>[2x]MEEPEEPADSGQSLVPVYIYSPEYVSMCDSLAKIPKRASMVHSLIEAYALHKQMRIVKPKVASMEEMATFHTDAYLQHLQKVSQEGDDDHPDSIEYGLGYDCPATEGIFDYAAAIGGATITAAQCLIDGMCKVAINWSGGWHHAKKDEA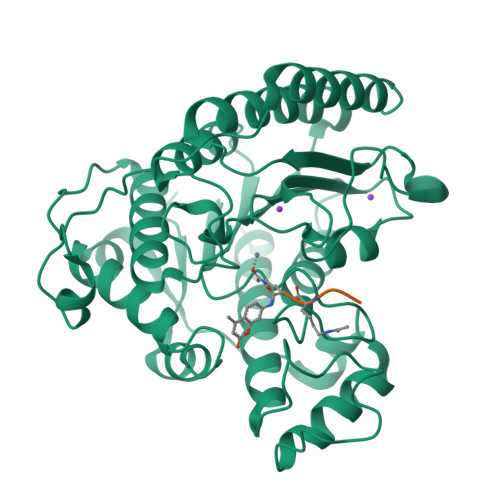SGFCYLNDAVLGILRLRRKFERILYVDLDLHHGDGVEDAFSFTSKVMTVSLHKFSPGFFPGTGDVSDVGLGKGRYYSVNVPIQGGIQDEKYYQICESVLKEVYQAFNPKAVVLQLGADTIAGDPMCSFNMTPVGIGKCLKYILQWQLATLILGGGGFNLANTARCWTYLTGVILGKTLSSEIPDHEFFTAYGPDYVLEITPSCRPDRNEPHRIQQILNYIKGNLKHVVIEGRGSHHHHHH>MAFCFGSFFSKYASSKSGSQARYRFLHSSAKIAAGATGALLLGGATVALCYFPSGRKVTEAPPFDVNSLRRDIEEILSEDMSKGPLFVRLAWHEAGSWDCRKKDGSPNSASMRFHPECSYA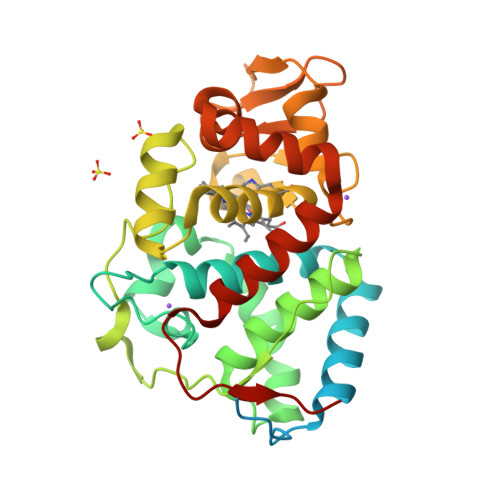GNKGLDKGRNALESLKKKYPKISYADLWSFAAVVSIEAMGGPEIPWRWGRVDAKDGSVCGPDGRLPDASRMQDHVRDVFSRLGFNDEETVALIGAHTCGECHLENTGYVGPWTHDKYGFDNSFFTELFGNEWMLNPNVKKMQFMDKTTNRLMMLPADVSILLDDKYRSIAKKYADDNDYFCNAFSKAYQKLLEVGTTDLKSLPAESK[2x]> SVPIVSAWEKGMEAARALMDKYHVDNDLKANFKLLPDQVEALAAVCKTWLNEEHRGLQLTFTSNKTFVTMMGRFLQAYLQSFAEVTYKHHEPTGCALWLHRCAEIEGELKCLHGSIMINKEHVIEMDVTSENGQRALKEQSSKAKIVKNRWGRNVVQISNTDARCCVHDAACPANQFSGKSCGMFFSEGAKAQVAFKQIKAFMQALYPNAQTGHGHLLMPLRCECNSKPGHAPFLGRQLPKLTPFALSNAEDLDADLISDKSVLASVHHPALIVFQCCNPVYRNSRAQGGGPNCDFKISAPDLLNALVMVRSLWSENFTELPRMVVPEFKWSTKHQYRPV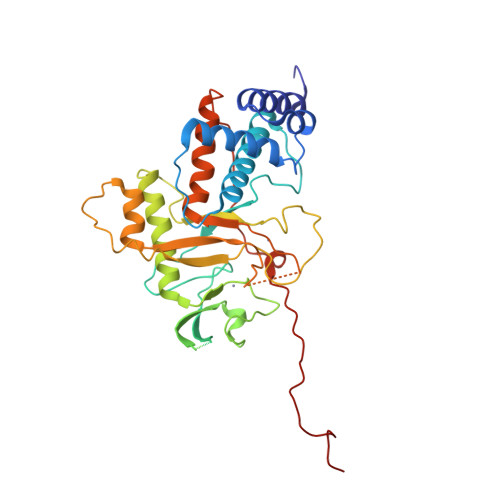SLPVAHSDARQNPFDF>MNRKWEAKLKQIEERASHYERKPLSSVYRPRLSKPEEPPSIWRLFHRQAQAFNFVKSCKEDVHVFALECKVGDGQRIYLVTTYAEFWFYYKSRKNLLHCYEVIPENAVCKLYFDLEFNKPANPGADGKKMVALLIEYVCKALQELYGVNCSAEDVLNLDSSTDEKFSRHLIFQLHDVAFKDNIHVGNFLRKILQPALDLLGSEDDDSAPETTGHGFPHFSEAPARQGFSFNKMFTEKATEES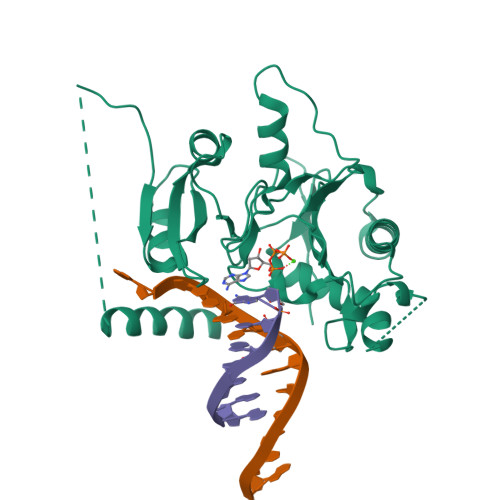WTSNSKKLERLGSAEQSSPDLSFLVVKNNMGEKHLFVDLGVYTRNRNFRLYKSSKIGKRVALEVTEDNKFFPIQSKDVSDEYQYFLSSLVSNVRFSDTLRILTCEPSQNKQ[2x]>[4x]GAMHALGHCCTVVTTRGPSHWLLLLDTHLGTLPGFKVSAGRGLPAAEVYFEAGPRVSLSRTDATIVAVYQSILFQLLGPTFPASWTEIGATMPHNEYTFPRFISNPPQFATLAFLPLLSPTSPLDLRALMVTAQLMCDAKRLSDEYTDYSTLSASLHGRMVATPEISWSLYVVLGIDSTQTSLSYFTRANESITYMRYYATAHNIHLRAADLPLVAAVRLDDLKDHQIPAPGSWDDLAPKLRFLPPELCLLL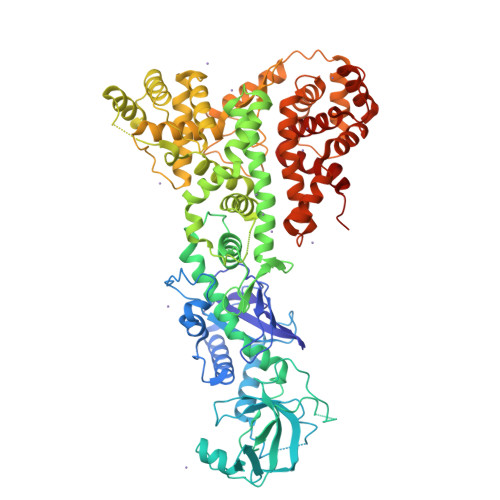PDEFDLIRVQALQFLPEIAKHICDIQNTICALDKSFPDCGRIGGERYFAITAGLRLDQGRGRGLAGWRTPFGPFGVSHTDVFQRLELLGDAVLGFIVTARLLCLFPDASVGTLVELKMELVRNEALNYLVQTLGLPQLAEFSNNLVAKSKTWADMYEEIVGSIFTGPNGIYGCEEFLAKTLMSPEHSKTVGSACPDAVTKASKRVCMGEAGAHEFRSLVDYACEQGISVFCSSRVSTMFLERLRDIPAEDMLDWYRLGIQFSHRSGLSGPGGVVSVIDIMTHLARGLWLGSPGFYVEQQTDKNESACPPTIPVLYIYHRSVQCPVLYGSLTETPTGPVASKVLALYEKILAYESSGGSKHIAAQTVSRSLAVPIPSGTIPFLIRLLQIALTPHVYQKLELLGDAFLKCSLALHLHALHPTLTEGALTRMRQSAETNSVLGRLTKRFPSVVSEVIIESHPKIQPDSKVYGDTFEAILAAILLACGEEAAGAFVREHVLPQVVADA Parechoviruses, including *Parechovirus A* that infects humans as well as *Parechovirus B* (formerly Ljungan virus) and *Parechovirus C* (formerly Sebokele virus) that infect rodents, belong to a group of picornaviruses whose 2A proteins, instead of being proteases, contain a conserved H-box and NC-motif and are homologous to a small cellular lipid-modifying enzyme (PLAAT3) that acts as a host factor, enabling the picornavirus life cycle. Despite the common evolutionary origin, 2A^H/NC^ proteins and PLAAT3 have no conserved function, as the active site of the viral proteins cannot support catalysis. Our structural analysis has shown that the topological rearrangement first observed in HPeV1 and leading to the apparent destruction of the active site configuration of the enzyme is indeed a general feature of *Parechovirus* 2A proteins. The C-terminal α5 region, which is a unique C-terminal extension so far only observed in *Parechovirus* 2A proteins, clearly plays a central role in determining the order of oligomerization as well as other correlated and sometimes far-reaching structural rearrangements.

Intrigued by this observed disorder in the C-terminal region of the *Parechovirus B* structures and its apparent influence on protein oligomerization, we decided to extend our structural characterization to the H/NC-motif type 2A_2_ of Sebokelevirus (SEBV1), the sole representative of *Parechovirus C*, which like *Parechovirus B* 2A_2_, exhibits shortened N- and C-termini compared to *Parechovirus A*. The structure of SEBV1-2A_2_ was determined to 1.56 Å resolution in space group P2_1_2_1_2 with two molecules in the asymmetric unit and was refined to 20.16% R_free_, no Ramachandran outliers, a Ramachandran Z-score of −0.40±0.53 and a Molprobity score of 1.16 (98^th^ percentile) ([Table tbl1]). All 134 residues could be modeled in both chains, and the final model includes an additional 5 residues at the N- and 7 residues at the C-terminus that were introduced during the cloning procedure, as well one ethylene glycol molecule, a tetraethylene glycol fragment and 256 water molecules. Overall, SEBV1-2A_2_ is similar to the LV 2A_2_ structures (3.70 Å over the full chain; 1.2 Å over the core 97 C_α_ residues), in SEBV1 however, the C-terminal α5 helix is well ordered (and extends to include two of the extra residues past the native protein boundaries) ([Fig fig1]). SEBV1-2A_2_ assembles into the same overall dimer configuration as HpeV1, despite having closer sequence identity with LV-2A_2_ ([Fig fig2]). In SEBV1-2A_2_, the C-terminal helix α5 folds back onto the globular domain, which positions it close to where α2 sits on HPeV1, and α2 shifts ∼7.5Å away from the interface.

>[2x]GPLGSPTMELVYKDRGFYKHYGVRVGNAIYHLDSQDILSTAITGQATFDKIEDDGCWLVSQVADLDYFTDKYVNSLVGTKHIFSATQNCETIARDVFGDSSMTQGRALGILGVILLSAGLLSLMAVPWDVSSLQQVYNQLTRAAAS> QDSTSDLIPAPPLSKVPLQQNFQDNQFHGKWYVVGLAGNRILRDDQHPMNMYATIYELKEDKSYNVTSVISSHKKCEYTIATFVPGSQPGEFTLGNIKS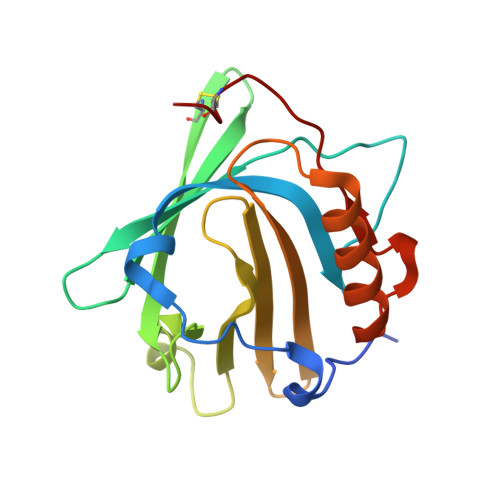YGDKTSYLVRVVSTDYNQYAVVFFKLAEDNAEFFAITIYGRTKELASELKENFIRFSKSLGLPENHIVFPVPIDQCIDG We identified two virulence pili independently critical to A. baumannii catheter-associated urinary tract infections, the chaperone-usher pathway pili Abp1 and Abp2. Further, their respective tip-adhesive proteins, the adhesins Abp1D and Abp2D, make use of large, distally oriented binding pockets to adhere to glycoproteins like fibrinogen, a wound-healing protein important in CAUTI pathogenesis. We demonstrate that Abp1D and Abp2D RBDs are structurally similar, and each binds fibrinogen and other relevant host glycoproteins important in CAUTI and other infections. These proteins share a common binding mechanism, using a large, distally oriented, and flexible pocket that recognizes a complex glycan receptor.

We next inverted the side chain charge at position 86, creating R86E, to attempt to actively repel adherence. This R86E mutation abolished Abp2D binding to BSM. To assess whether the reduced-binding R86E mutation modulates the anterior loop opening dynamics, we crystallized the Abp2DRBD R86E protein, resulting in a cuboidal crystal, which was solved at 1.9 Å resolution (8 DKA). The electron density of the anterior loop is sparse, starting at position 86, even though the rest of the protein is well-modeled. This indicates that the loop is flexible and oriented in different conformations between different molecules throughout the crystal. However, we were able to model the R86E anterior loop, finding that it is displaced dramatically up and into the binding pocket by 11.6 Å relative to the structure solved for Abp2DRBD WT. Consistent with our hypothesis, the R86E mutant ensemble is characterized by a greater diversity of open and closed distances. R86E also exhibits an increase in the total number of heterogeneous conformations, indicating that this anterior binding pocket loop is destabilized by this mutation. Our findings indicate that the R86E null binding phenotype may in part be caused by the flexibility in the anterior loop in addition to the charge difference resulting from arginine to glutamate side mutation. For R86E, the electrostatic consequences of the side chain charge inversion, necessary to eliminate binding at this position, could be contributing to the flexibility of the anterior loop motif. R86E mutations in both Abp1DRBD and Abp2DRBD uniformly decrease the binding of the protein construct to each of the tested glycoproteins.

> YCTLSSGFTTVDISMAVGRVVVRPSDPVGKILRKATFPINPNGSTLRCTSYSDTITAALTQNYPLSPLGNSIYSTNIPGIGIRLYEEAENATNFSGYYPYTRSLTPGTTYNLAQGYFVVEIVKTADQTGSGTLVPGLYSRYYVNGHMDRPFLTSTVYGNAITIASSSHHHHHH> MSSWDRFDTPWDSIIDESTWEHYTFKYDASFEAFSSMEV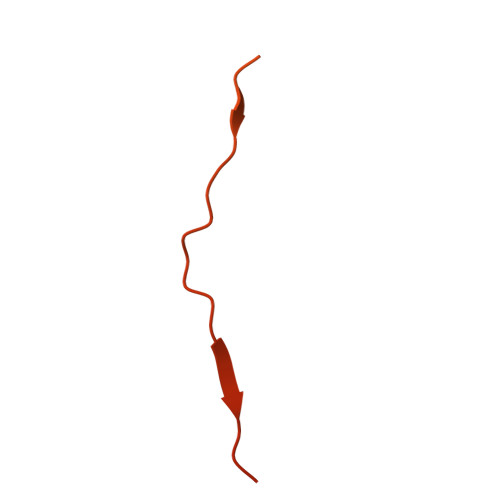DEDLTITVSVLFASTSDNTVTVGQVLGLTMDNRAGSYFGAGSSWTSEAAVNNEAGSGFQSSHALQLSYSVEDGVISSFGSEAFCSFYNTVSFESSSDVQAAVNSLYNLDVLFSSGSGDSEQHYVVFGETASFESLAEHETSSQYITHVECMFNSVVEFEVKTYDWGRPVKPVGSDWSTDTPVVGVWVNEIYNGNKDWGES Improved proteomic analyses subsequently revealed that, in addition to syntrophins, α1D-ARs also interact with the multi-PDZ domain containing protein scribble (SCRIB); and that α1D-ARs are expressed as modular homodimers, with one α1D-AR protomer bound to SCRIB, the other to syntrophin, in all human cell lines examined to date. A defining structural characteristic of SCRIB includes the presence of four clustered PDZ domains in the C-terminal portion of the polypeptide. Herein, we employed a combination of biophysical, biochemical and cell-based approaches to acquire structural insights into the α1D-AR:PDZ protein complex. Together, our data implicate SCRIB PDZ domains 1 and 4 as the primary anchor sites for the α1D-AR. Without significant expression of necessary PDZ proteins, α1D-ARs are retained intracellularly and produce weak functional responses, suggesting this protein:protein interaction site has the potential for pharmacological modulation.

Our model identified D571α1D-AR:R1110PDZ4 of the carboxylate binding loop and T570α1D-AR:H1170PDZ4 of α-helix B as possible α1D-CT PDZ ligand interaction sites within SCRIB PDZ4. SCRIB PDZ domain sequence alignment revealed that R1110, but not H1170, is unique to PDZ4, suggesting that this residue may be responsible for the specificity of α1D-AR to PDZ4. In support of our structural prediction, purified PDZ4 harboring either R1110G or H1170A mutations ablates α1D-CT binding. However, the structural role of R1110 is unknown. A superposition of the R1110G mutant with WT PDZ4 reveals a 4.5 Å shift of the carboxylate binding loop. We predict this shift creates steric hindrance that prevents the interaction between I572α1D-AR and PDZ4. Previous studies have found PDZ ligand:PDZ domain interactions are dictated by interactions of the C-terminal residue of the PDZ ligand. Finally, we demonstrate that SCRIB R1110PDZ4 serves as a unique α1D-CT interface site that could be targeted to modulate α1D-AR pharmacodynamics. Thus, targeting SCRIB PDZ4 may provide the highest opportunity to disrupt α1D-AR function without perturbing other SCRIB complexes.

> SHMLRELCIQKAPGEGLGISIRGGARGHAGNPRDPTDEGIFISKVSPTGAAGRDGRLRVGLRLLEVNQQSLLGLTHGEAVQLLRSVGDTLTVLVC> TCTCTACTGTGGATGAAC;> GAGTTCATCCT;> GGACAGTAGA;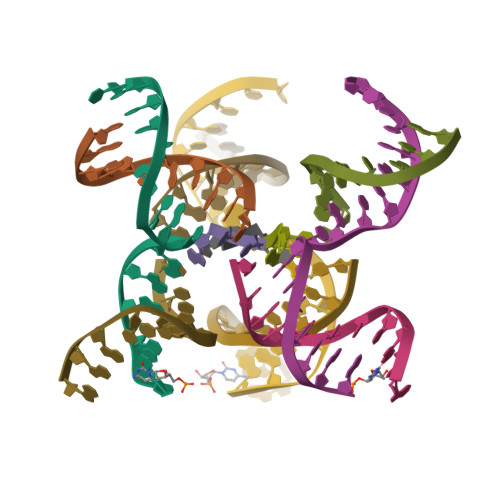> ACC> VLGKPQTDPTLEWFLSHCHIHKYPSKSTLIHQGEKAETLYYIVKGSVAVLIKDEEGKEMILSYLNQGDFIGELGLFEEGQERSAWVRAKTACEVAEISYKKFRQLIQVNPDILMRLSAQMARRLQVTSEKVGNL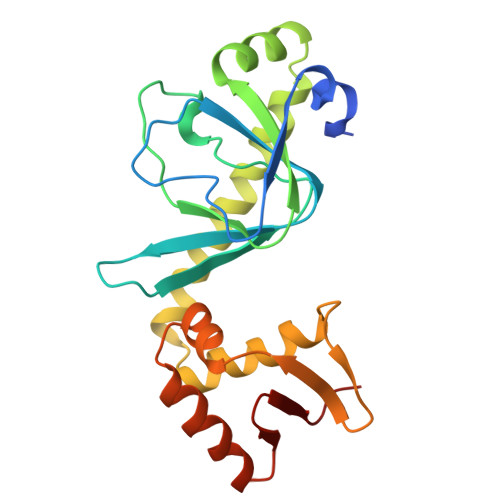AFLDVTGRIAQTLLNLAKQPDAMTHPDGMQIKITRQEIGQIVGCSRETVGRILKMLEDQNLISAHGKTIVVYGTR> MSTYEGRWKTVKVEIEDGIAFVILNRPEKRNAMSPTLNREMIDVLETLEQDPAAGVLVLTGAGEAWTAGMDLKEYFREVDAGPEILQEKIRREASQWQWKLLRMYAKPTIAMVNGWCFGGGFSPLVACDLAICADEATFGLSEINYGIPPGNLVSKAMADTVGHRQSLYYIMTGKTFGGQKAAEMGLVNESVPLAQLREVTIELARNLLEKNPVVLRAAKHGFKRCRELTWEQNEDYLYAKLDQSRLLDTEGGREQGMKQFLDDKSI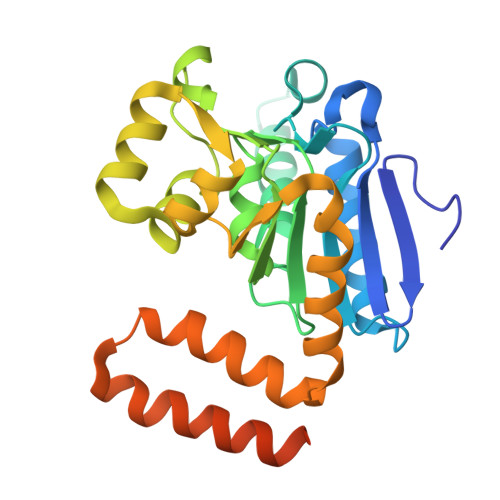KPGLQAYKR> LSEEQQHIIAILLDAHHKTYDPTYADFRDFRPPVRMDGSTGSVTLDLSPLSMLPHLADLVSYSIQKVIGFAKMIPGFRDLTSDDQIVLLKSSAIEVIMLRS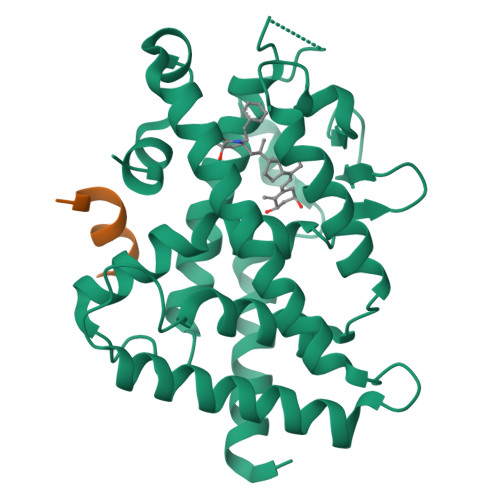NQSFTMDDMSWDCGSQDYKYDVTDVSKAGHTLELIEPLIKFQVGLKKLNLHEEEHVLLMAICIVSPDRPGVQDAKLVEAIQDRLSNTLQTYIRCRHPPPGSHQLYAKMIQKLADLRSLNEEHSKQYRSLSFQPENSMKLTPLVLEVFGN;> NHPMLMNLLK> AFDAFLKIDGIPGESSDDKHKDWIEIQSFAHKLEQPAQATASSAGGATAERVNHAAYEITHFLDKASPKIYEACCKGQHIKEITIELCRAGGDKVKYME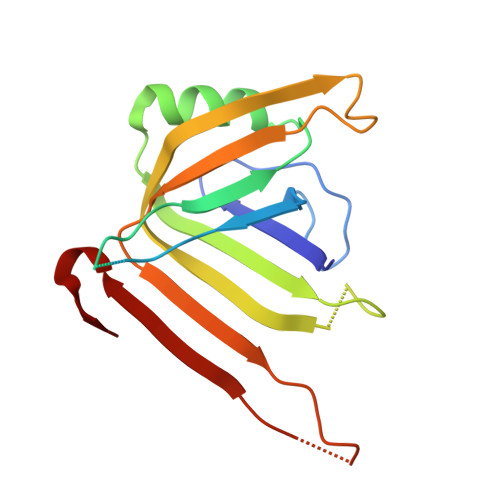IKMEQVLIAKVEPHGSANDNGFPSEKVSFTYGKIKWTYTQQKRADGAGGGNVSSGWDLTANKAI Flavin-dependent halogenases (FHals) play an essential role in the regioselective halogenation of natural products such as chloramphenicol, vancomycin, or cryptophycin. Only halide salts, oxygen, and the cofactor FADH2 are required for regioselective halogenation. We were able to show that the gene product forms an active enzyme and catalyses the halogenation of free indole in C3 position. Interestingly, BrvH possesses an intriguing selectivity for bromide over chloride in halogenation that, however, cannot be directly explained from the crystal structure.

The structure of apo BrvH without any bound ligands was determined to a resolution of 2.5 Å. There are two chains in the asymmetric unit with no major differences between the chains. In the crystal, it forms a dimer very similar to that of tryptophan halogenases like PrnA or RebH. BrvH was modelled nearly completely, except for a few terminal residues and residues 46–51, a loop involved in FAD binding that can adopt various conformations in other FHals and is disordered in apo BrvH. The substrate binding site is only partly conserved between BrvH and RebH. There are no equivalent residues in BrvH, as a short loop (residues 432–444) replaces its much longer counterpart in RebH (residues 440–467). As a consequence, the substrate binding site of BrvH is noticeably more open than that of tryptophan halogenases and the ε-amino group of the active site lysine K83 is directly accessible to the solvent. The lack of side chains to keep the amino and carboxy group of tryptophan in place could potentially explain why BrvH does not accept tryptophan as substrate. The openness of the substrate binding site and the absence of large non-polar patches–which would point to a variant B halogenase [14]–resemble the structure of MibH, a tryptophan halogenase that chlorinates tryptophan only when the latter is part of the enzyme’s cognate substrate peptide (deschloro NAI-107). The structure does not contain FAD and there is no halide bound at the assumed halide binding site, the amide nitrogens of T351 and S352 (T359 and G360 in RebH).

>GAMDEIDDPRIRSVVIVGGGTAGWMTAAALVQHFRTAPLKITVVESSDIGTIGVGEATIPTIRRFYGQLGLRDDDVMRATQATCKLGIRFLDWSGPGSDFIHPFGLYGQDVKGIGFHHYWLKQRRAGDAAPLAAYSLGAALAAGGKFTLPSPHPPSQLSVFDWALHLDAGLFAQHLRAYAEAGGCARIDARIRSVELRPEDGFVRALTLDDGREVEGDLFVDCSGFKGLVIGEALGVGFEDWGRWLPCDAAYAVQSENRPGDAPAPFTRVTARSAGWQWGIPLRHRAGNGLVFSSAHLSDDQALAELMPHLLGDPLTEPRRIPFRPGRRSQAWAKNCVAIGLSSGFLEPLESTSIALIETGIERLKALFPDRRFAQPILDEFNDQTAREMERVRDFIILHYKLNRRTDTDFWRDCREMPVPETLERKIALWTARGQFVRYRWEMFHPASWLAIYDGFGLYPDHHDPAVDAMDPAYLARSLAEMRANIADLVARTPEHAQFLAGLDPAASAA[2x]>SHMKITAINVFQVDLPLREGRYSWSNGNFVEVFDSTVVEIETDEGLKGYAECCPLGSAYLPSYALGVRSGLQELAPHLIGKDPLNIGEINRVMDAALRGHPYAKAPIDIACWDLLGKATGQPLYTLLGGAAQDDVALYRAISQEAPEIMAKKIEGYAAEGYTKFQLKVGGDANDDINRIHATRSVLKKSDLLVADANTGWTRHEAARVVGAVSSLDVYIEQPCLTYEESVSIRRRTALPFVLDEVIDGPNTLVRGIAEDAMDCINLKISKVGGLTKAKLMRDLCIAHGIPMTIEDTWGGDIVTAAIAHLARSTPSEFTFSATDFNSYGTVDIAEGAPKR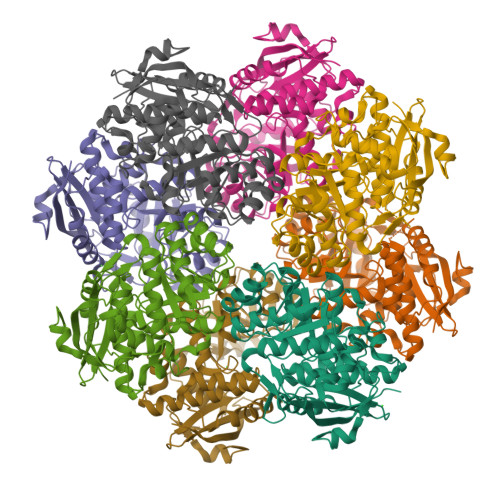VNGRMTTSDLPGLGITPIFDVLGEPVARYS[8x]> MLQVDIGSTSGKAGSVVSVPITFTNVPKSGIYALSFRTNFDPQKVTVASIDAG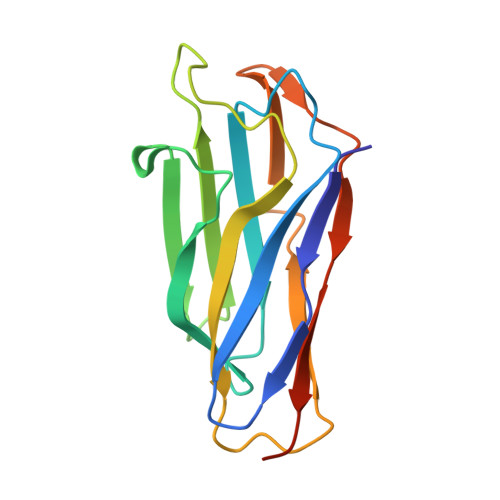SLIENASDFTTYYNNENGFASMTFEAPVDRARIIDSDGVFATINFKVSDSAKVGELYNITTNSAYTSFYYSGTDEIKNVVYNDGKIEVIALEHHHHHH>MSRLLVIGCGGVAQVAISKICQDSETFTEIMIASRTKSKCDDLKAKLEGKTSTKIETAALDADKVEEVIALIGSYKPEAVLNVALPYQDLTIMDACLATGVHYIDTANYEAEDTEDPEWRAIYEKRCKELGFTAYFDYSWQWAYQEKFKEAGLTALLGSGFDPGVTSVFSAYALKHYFDEIHYIDILDCNGGDHGYPFATNFNPEINLREVSAPGSYWEDGKWVEVEAMSIKREYDFPQVGQKDMYLLHHEEIESLAKNIPGVKRIRFFMTFGQSYLTHMKCLENVGLLRTDTINFNGQEIVPIQFLKALLPDPASLGPRTVGKTNIGCIFTGVKDGVEKTIYIYNVCDHQECYAEVGSQAISYTTGVPAMIGTKLVMNGTWKQAGVYNLEELDPDPFMEALNEYGLPWVVVENPQMV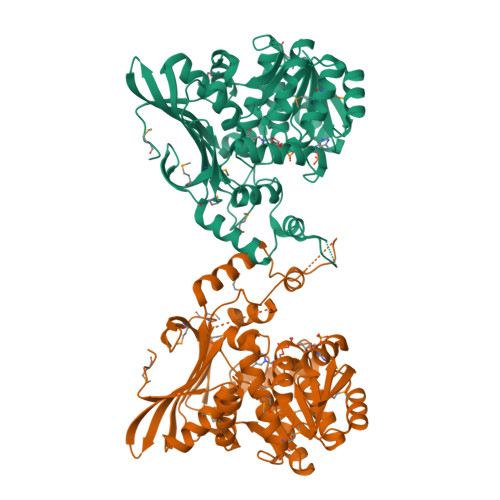DLEHHHHHH[2x]>MKKRLTESQFQEAIQGLEVGQQTIEIARGVLVDGKPQATFATSLGLTRGAVSQAVHRVWAAFEDKNLPEGYARVTAVLPEHQAYIVRKWEADAKKKQET[3x];> MKKRLTESQFQEAIQGLEVGQQTIEIARGVLVDGKPQATFATSLGLTRGAVSQAVHRVWAA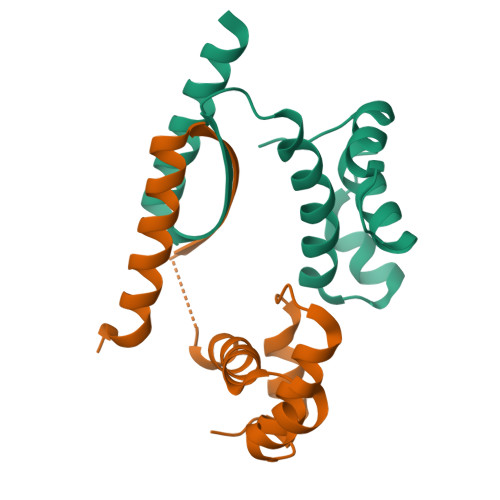FEDKNLPEGYARVTAVLPEHQAYIVRKWEADAKKKQETKR> MVNISDFFGKNKKSVRSSTSRPTRQVGSSKPEVIDLDTESDQESTNKTPKKMPVSNVIDVSETPEGEKKLPLPAKRKASSPTVKPASSKKTKPSSKSSDSASNITAQDVLDKIPSLDLSNVHVKENAKFDFKSANSNADPDEIVSEIGSFPEGKPNCLLGLTIVFTGVLPTLERGASEALAKRYGARVTKSISSKTSVVVLGDEAGPKKLEKIKQLKIKAIDEEGFKQLIAGMPAEGGDGEAAEKARRKLEEQHNIATKEAELLVKKEEERSKKLAATRVSGGHLERDNVVREEDKLWTVKYAPTNLQQVCGNKGSVMKLKNWLANWENSKKNSFKHAGKDGSGVFRAAMLYGPPGIGKTTAAHLVAQELGYDILEQNASDVRSKTLLNAGVKNALDNMSVVGYFKHNEEAQNLNGKHFVIIMDEVDGMSGGDRGGVGQLAQFCRKTSTPLILICNERNLPKMRPFDRVCLDIQFRRPDANSIKSRLMTIAIREKFKLDPNVIDRLIQTTRGDIRQVINLLSTISTTTKTINHENINEISKAWEKNIALKPFDIAHKMLDGQIYSDIGSRNFTLNDKIALYFDDFDFTPLMIQENYLSTRPSVLKPGQSHLEAVAEAANCISLGDIVEKKIRSSEQLWSLLPLHAVLSSVYPASKVAGHMAGRINFTAWLGQNSKSAKYYRLLQEIHYHTRLGTSTDKIGLRLDYLPTFRKRLLDPFLKQGADAISSVIEVMDDYYLTKEDWDSIMEFFVGPDVTTAIIKKIPATVKSGFTRKYNS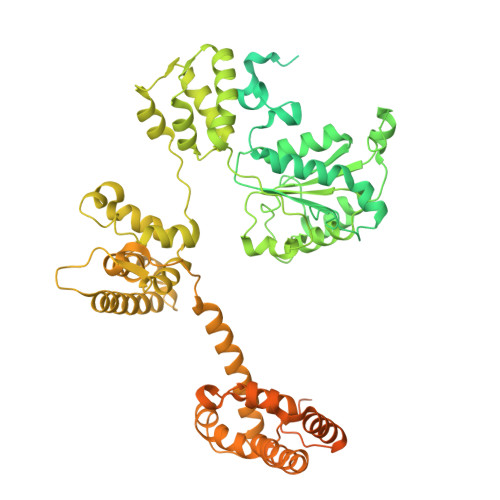MTHPVAIYRTGSTIGGGGVGTSTSTPDFEDVVDADDNPVPADDEETQDSSTDLKKDKLIKQKAKPTKRKTATSKPGGSKKRKTKAGLNENLYFQGGGDYKDDDDKDYKDDDDKDYKDDDDKGGKDHLIHNVHKEEHAHAHNK> MKSSHHHHHHENLYFQSNAELQPQFNEFLANIRPTDTQKEDWKSGARTLRERLKNFEPLKEIVVSTFLQGSIRRSTAIRPLGDKRPDVDIVVVTNLDHTRMSPTDAMDLFIPFLEKYYPGKWETQGRSFGITLSYVELDLVITAIPESGAEKSHLEQLYKSESVLTVNSLEEQTDWRLNKSWTPNTGWLSESNSAQVEDAPASEWKAHPLVLPDREKNEWGRTHPLAQIRWTAEKNRLCNGHYINLVRAVKWWRQQNSEDLPKYPKGYPLEHLIGNALDNGTTSMAQGLVQLMDTFLSRWAAIYNQKSKPWLSDHGV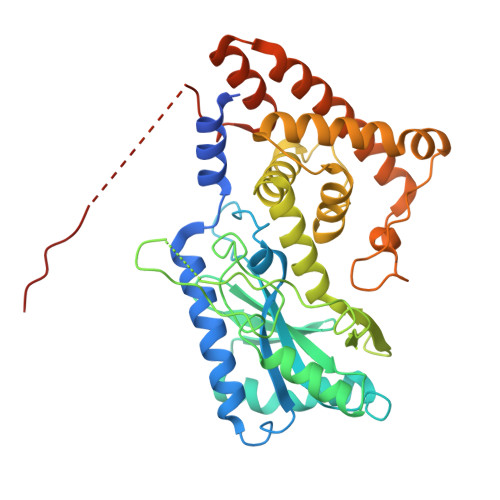AEHDVMARLTAEDFCSFYEGIASAAEIARNALASEEPQESAQLWRQLFGSKFPLPGPQGGDRNGGFTTPSKPAEPQKTGRFA>[2x]SANSGCKDVTGPDEESFLYFAYGSNLLTERIHLRNPSAAFFCVARLQDFKLDFGNSQGKTSQTWHG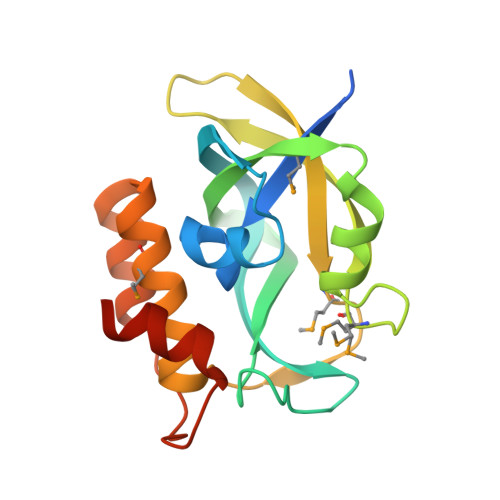GIATIFQSPGDEVWGVVWKMNKSNLNSLDEQEGVKSGMYVVIEVKVATQEGKEITCRSYLMTNYESAPPSPQYKKIICMGAKENGLPLEYQEKLKAIEPNDYTGKVSEEIEDIIKKGETQTL>MKSRIIVRTSFDAAHAVKVGDHWEDVHGHTFFLEVAIEGEIKNGYVMDFLELRKIVEEITKELDHRNLNNIFENPT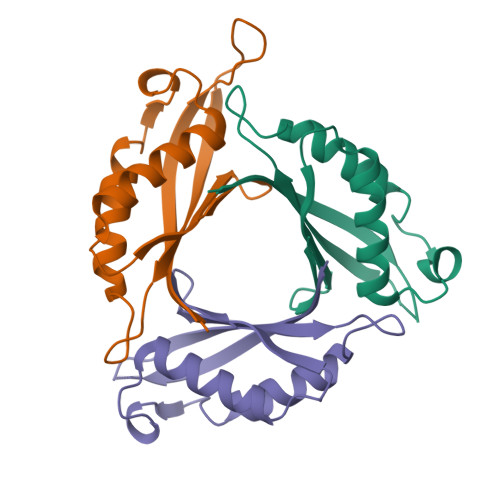TENIALWIGERIRDKLPPYVKLKRVVLWEGKDNGVELEW[3x]>MTTYLEFIQQNEERDGVRFSWNVWPSSRLEATRMVVPVAALFTPLKERPDLPPIQYEPVLCSRTTCRAVLNPLCQVDYRAKLWACNFCYQRNQFPPSYAGISELNQPAELLPQFSSIEYVVLRGPQMPLIFLYVVDTCMEDEDLQALKESMQMSLSLLPPTALVGLITFGRMVQVHELGCEGISKSYVFRGTKDLSAKQLQEMLGLSKVPLTQATRGPQVQQPPPSNRFLQPVQKIDMNLTDLLGELQRDPWPVPQGKRPLRSSGVALSIAVGLLECTFPNTGARIMMFIGGPATQGPGMVVGDELKTPIRSWHDIDKDNAKYVKKGTKHFEALANRAATTGHVIDIYACALDQTGLLEMKCCPNLTGGYMVMGDSFNTSLFKQTFQRVFTKDMHGQFKMGFGGTLEIKTSREIKISGAIGPCVSLNSKGPCVSENEIGTGGTCQWKICGLSPTTTLAIYFEVVNQHNAPIPQGGRGAIQFVTQYQHSSGQRRIRVTTIARNWADAQTQIQNIAASFDQEAAAILMARLAIYRAETEEGPDVLRWLDRQLIRLCQKFGEYHKDDPSSFR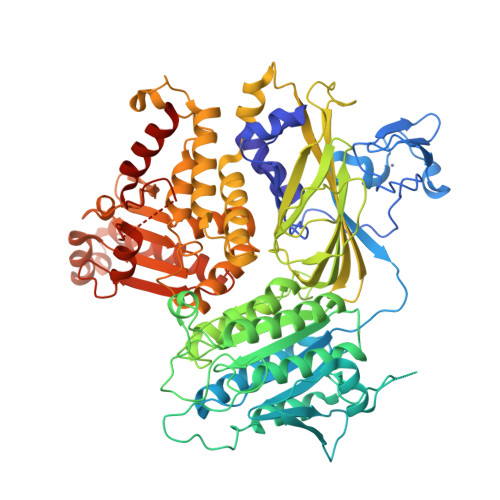FSETFSLYPQFMFHLRRSSFLQVFNNSPDESSYYRHHFMRQDLTQSLIMIQPILYAYSFSGPPEPVLLDSSSILADRILLMDTFFQILIYHGETIAQWRKSGYQDMPEYENFRHLLQAPVDDAQEILHSRFPMPRYIDTEHGGSQARFLLSKVNPSQTHNNMYAWGQESGAPILTDDVSLQVFMDHLKKLAVSSAA[2x];> GPRPLPPP> MSKGKKRSGARPGRPQPLRGTKGKRKGARLWYVGGQQ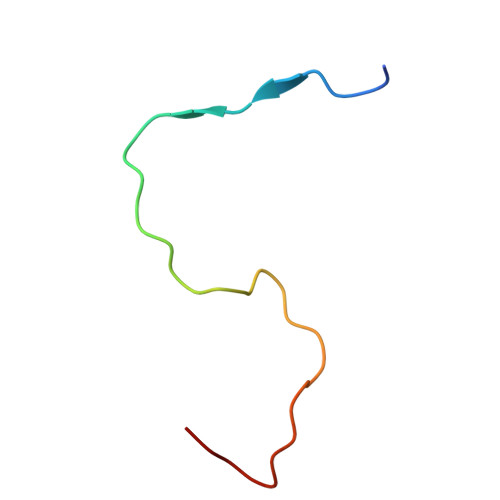F>[2x]MAHFHYSSLLAQPQINKEIKNEDGVDIDRTLVAKQSIVKFELKTEALTAGRPKTTSFVLVDPLPTGYKFDLDATKAASTGFDTTYDEASHTVTFKATDETLATYNADLTKPVETLHPTVVGRVLNDGAT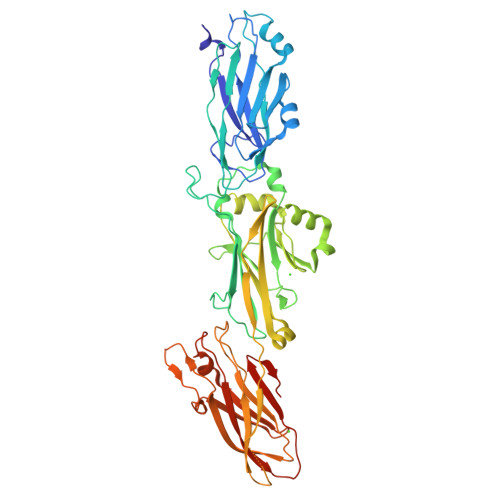YTNNFTLTVNDAYGIKSNVVRVTTPGKPNDPDNPNNNYIKPTKVNKNKEGLNIDGKEVLAGSTNYYELTWDLDQYKGDKSSKEAIQNGFYYVDDYPEEALDVRPDLVKVADEKGNQVSGVSVQQYDSLEAAPKKVQDLLKKANITVKGAFQLFSADNPEEFYKQYVATGTSLVITDPMTVKSEFGKTGGKYENKAYQIDFGNGYATEVVVNNVPKITPKKDVTVSLDPTSENLDGQTVQLYQTFNYRLIGGLIPQNHSEELEDYSFVDDYDQAGDQYTGNYKTFSSLNLTMKDGSVIKAGTDLTSQTTAETDATNGIVTVRFKEDFLQKISLDSPFQAETYLQMRRIAIGTFENTYVNTVNKVAYASAAALEHHHHHH>[2x]AMRQCAIYGKGGIGKSTTTQNLVAAL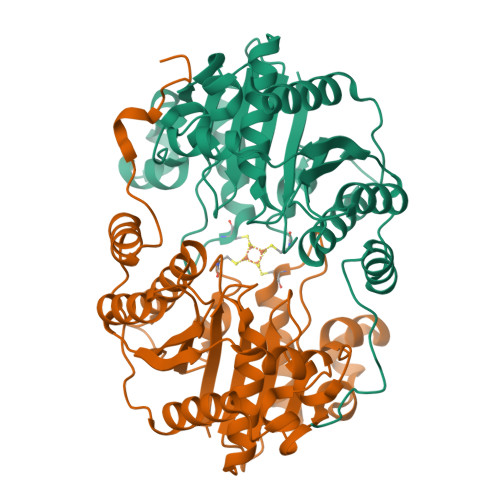AEMGKKVMIVGCDPKADSTRLILHSKAQNTIMEMAAEAGTVEDLELEDVLKAGYGGVKCVESGGPEPGVGCAGRGVITAINFLEEEGAYEDDLDFVFYDVLGDVVCGGFAMPIRENKAQEIYIVCSGEMMAMYAANNISKGIVKYANSGSVRLGGLICNSRNTDREDELIIALANKLGTQMIHFVPRDNVVQRAEIRRMTVIEYDPKAKQADEYRALARKVVDNKLLVIPNPITMDELEELLMEFGIMEVEDESIVGKTAEEV>[4x]MSPNRFLLCVCILGLIAGGAAKVQYALTIPALLKSGETQRACVNLIGYHQPLALSVVLEHQRVNISIFSEKVQPPHYFKCNKFMVPTVITNAPDFVTLSVSGGGEDIKDRKAVVIAPLNTICLIQMDKPVYKPGCKVRFRLISLNTMLLPISEKYTAVYLEDPSGSRIAQWQNQESVGGVVQLEFPLISDAAPGSYTITAEGESCESARQGFTVDEYILPRFSVIVDPPNTISILDDILTLNVSAIYTYGQPVPGSVTIKCCREASSYYGRKGNCFKGNRGICTNITGELGPDGAFYGVVSLLPFQMGQSGFQMSLGVALTVTEEGTGIQVTHQFFIMITSQLATLIFDYDALKEFYKRGIPYLVKVILTDANDNPMANEQVEVELAGKTIGAVLTDKEGRAEYAIDTSSFVQENFTVVVSYENPHQCYYTEWEGPDFPTAQHFVMRFYSET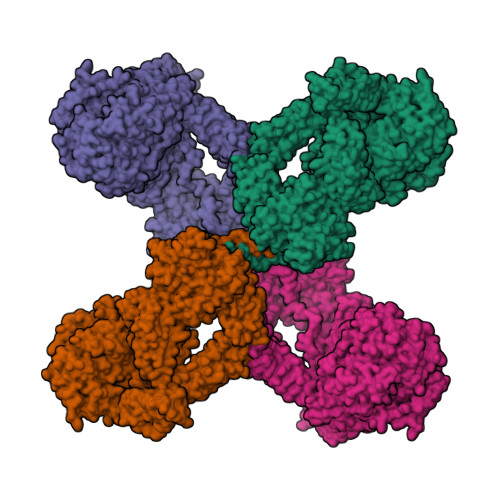GSFLDIQGSSVELNCGQVHNISVRYILSLDGMGEGATTATFYYLAMSRAKIVQHGQRDVHLNQSKSGLFNIGLNVTSDLAPGAELIVYCILDLELIADTISLDIEKCFQNQVSLSFSDDLGPTASNVSLNLSAAPGSLCGVKVIDSSLLLINPYESLSASGVYYSIPYLSLFGYNYGGFNLEEPEPPCEDPNTVIFCKGRYYLPVSSSTEGDTYQNLRRVGLVLGTSSKIRKPVVCGMEAKFSVPRKSSGESDFGSSLSNGHVETLRKNFSETFLWRLVSVDSEGQNTITETVPDTITKWQGSMFCVSEKEGFGITKYSANFTSFLPFFVELSLPYSLTREEILVMKAFVSNYLEECIKIIVTLQPSADFEVIPQDVKQDQCICSGGRSSYSWNIIASSLGRISFIVSAETTHIGASCDGPSDQSQSTRKDTVIQTILVQPEGIRKEETSSNLVCVEDSNVEMPINLTLPENIVQGSASAFVTFVGDVLGLPLSNLQNLLQMPYGCGEQNLARMAPIPYVLEYLNNTNQLTDELLQTAVQFLNEGYYRQLRYKLPSGAYDAFWSSPSDGSSWLSAYTFKTFEKAKKYIYVDGKIQQQTLLYLQTSQKLDNGCFKAEGNLFMRQCGQERDLCFTAYLAIALLESNYSSGMTLLDDALGCLEAAMSSASTLYFKSYTVYVFTLVQNWEIRNTLLNELKSKVVSERGTLHWEREDKLGQEGIPLYYPNYSPAEVEITAYMLLSIAKGSDPTHDDLTYMAQISVWLIQQQNSYGGFRSTQDTVVALQALAFYAQLLFKSNAHHNVFLRSEYGDVGQLNLSEHNRLVVQRLQLPEVSGNYSISINGTGCCLVQSTIRYNIPVPKENSAFYVAADSVSKNCLNGVAYTITITVSVSYRGLRNETNMVIIDIQMLSGYQADYPSLRQLENSQQVSKTEEQDNHVFLYLNAVPLKTIQLSFKVLIGSRVLNVKSASVYVYDYYETGENGFASYSQPC>VEGRFQLVAPYEPQGDQPQAIAKLVDGLRRGVKHQTLLGATGTGKTFTISNVIAQVNKPTLVIAHNKTLAGQLYSELKEFFPHNAVEYFVSYYDYAQPEAYVPQTDTYIEKDAKINDEIDKLRHSATSALFERRDVIIVASVSCIYGLGSPEEYRELVVSLRVGMEIERNALLRRLVDIQYDRNDIDFRRGTFRVRGDVVEIFPASRDEHCIRVEFFGDEIERIREVDALTGEVLGEREHVAIFPASHFVTREEKMRLAIQNIEQELEERLAELRAQGKLLEAQRLEQRTRYDLEMMREMGFCSGIENYSRHLALRPPGSTPYTLLDYFPDDFLIIVDESHVTLPQLRGMYNGDRARKQVLVDHGFRLPSALDNRPLTFEEFEQKINQIIYVSATPGPYELEHSPGVVEQIIRPTGLLDPTIDVRPTKGQIDDLIGEIRERVERNERTLVTTLTKKMAEDLTDYLKEAGIKVAYLHSEIKTLERIEIIRDLRLGKYDVLVGINLLREGLDIPEVSLVAILDADKEGFLRSERSLIQTIGRAARNANGHVIMYADTITKSMEIAIQETKRRRAIQEEYNRKHGIVPRTVKKEIRDVIRATYAAEETEMYEAKPAAAMT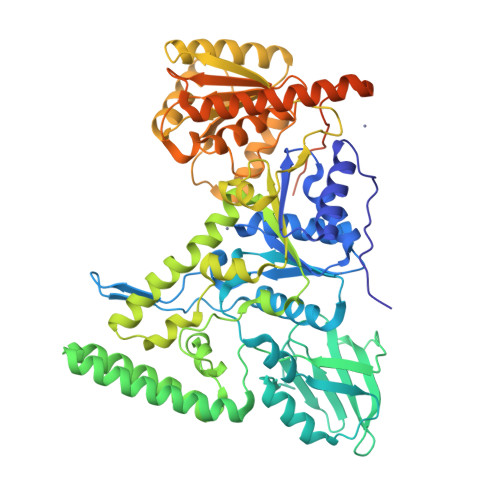KQEREELIRTLEAEMKEAAKALDFERAAQLRDIIFELKAEG[2x]Bacterial fibrillar adhesins are specialized extracellular polypeptides that promote the attachment of bacteria to the surfaces of other cells or materials. The fibronectin (Fn)‐binding fibrillar adhesin CshA, and its paralogue CshB, play important roles in host colonization by the oral commensal and opportunistic pathogen Streptococcus gordonii. The Streptococcus gordonii (S. gordonii) fibrillar adhesin cell surface hydrophobicity protein A (CshA) is an ∼259 kDa cell wall anchored polypeptide that confers fibronectin (Fn)‐binding properties to this bacterium. CshA comprises an N‐terminal “nonrepeat” (NR) region, which houses the adhesive CshA_NR2 domain, fused to a stalk‐forming “repeat region” (RR), incorporating 17 sequentially arrayed ~100 amino acid domains.

To further advance our understanding of Csh adhesins, we next sought to elucidate the X‐ray crystal structure of the NR2 domain of the CshA paralogue CshB (residues 211–528 of the full‐length polypeptide). Despite repeated efforts, only the dimeric form of CshB_NR2 proved amenable to crystallization. The crystal structure of CshB_NR2 reveals a strand‐swapped homodimer, wherein residues 442–528 of each monomer are buried in the central core of the associated dimer partner. The exchanged region comprises β‐strands 12–14 of each polypeptide chain. Monomeric CshB_NR2 adopts an overall fold equivalent to that of CshA_NR2, with a Cα root‐mean‐square deviation (RMSD) between the two structures of 1.0 Å. The CshB_NR2 fold comprises a β‐sandwich core formed from two antiparallel β‐sheets, one of eight β‐strands and the other of six β‐strands. The periphery of the β‐sandwich is decorated with six α‐helices, which are located between strands β3/β4 (α1 and α2), β9/β10 (α3, α4, and α5) and after β14 (α6). In contrast to previous crystallographic studies of CshA_NR2, electron density was observed corresponding to the CshB_NR2 polypeptide chain beyond the final β‐strand of the protein (β14). This density corresponds to an extended loop punctuated by a short α‐helix (α6), which traverses the connecting loops between β6/β7, β8/β9, β10/β11, and β12/β13, and occupies a groove formed by the packing of α1 against the larger of the two β‐sheets. The CshB_NR2‐binding pocket is appreciably less negatively charged, predominantly as a consequence of the substitution of residues Asp300, Asp337, and Asp338 in CshA_NR2 with tyrosine (Tyr288), methionine (Met326) and asparagine (Asn327), which occupy equivalent positions in CshB_NR2.

> WLDFSDSASWKNLDQRGGLKVGTTFTKEISPGYVVTLTVKELKPFNSTEIYKKRVAGTATEGTYDPDAENGFLTSAPYYGKTPPPSVTGAAQNEWTTIRDQGFNTQKRKTQLVYPMNSTNWGVKFDIEATYLGKRVAPTVVMADGEDANPGEFAIFTTNGTGWEYMGEWKMKSPAKEAYNVITKKMLDDEDVKRRGLLILKDKSVDWYKYLSPDTVTGGLGSQVFGPNRSNERTVPVVMTRGASEVGFYVASSGQQAMMMGFLVVAVSDAPESYGEAFHTISTRDSVTNDPINQPYLGTTPADIDVESSNDWVLDDKK> MLNIGDLLGSTPAKDQACSRTCESQFCTIAPLLRYGKYCGILYSGCPGERPCDALDACCMVHDHCVDTHNDDYLNTMCNENLLSCID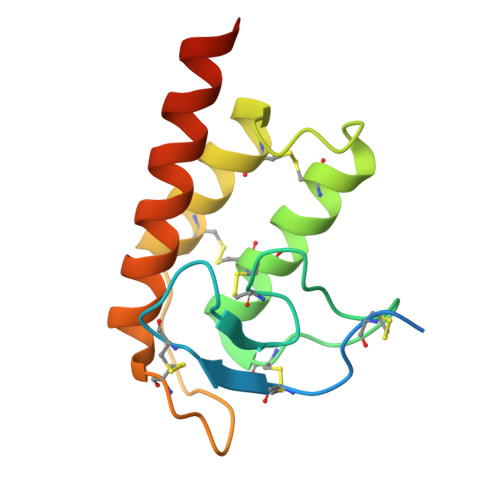RVSGATFPGNKCNVGQTASVIRGVIETAVFAGKILHKRDDGQ>MSAASWSHPQFEKMSRDEVEALIQEVLEVYPEKAKKDRAKHLAVNDQSVEQSKKCITSNKKSLPGVMTIRGCAYAGSKGVVWGPIKDMIHISHGPVGCGQYSRAGRRNYYIGTTGVNAFVTMNFTSDFQEKDIVFGGDKKLAKLIDEIETLFPLNKGISVQSECPIGLIGDDIEAVAKQKSAELGKTVVPVRCEGFRGVSQSLGHHIANDAVRDWVLSKRDDDDSFESTPYDVAIIGDYNIGGDAWSSRILLEEMGLRVVAQWSGDGTISEMELTPKVKLNLVHCYRSMNYISRHMEEKYGIPWMEYNFFGPTKTIESLRKIAAQFDESIQAKCEEVIAKYKPEWEAVIAKYRPRLEGKRVMLYVGGLRPRHVIGAYEDLGMEVVGTGYEFAHNDDYDRTIKEMGNATLLYDDVTGYEFEEFVKKVKPDLIGSGIKEKYIFQKMGIPFRQMHSWDYSGPYHGFDGFAIFARDMDMTLNNPCWKKLQAPWKKAESEAEAVAASA[2x];>MSQQVDNIKPSYPLFRDEEYKDMLAKKRDNFEEKHPQEKIDEVFQWTTTEEYQELNFQREALTVNPAKACQPLGAVLCALGFEKTMPYVHGSQGCVAYFRSYFNRHFKEPISCVSDSMTEDAAVFGGQQNMKDGLENCKAIYKPDMIAVSTTCMAEVIGDDLNAFINNSKKEGHIPEEFPVPFAHTPSFVGSHTTGWDNMFEGIARYFTLNYMEDKEVGSNGKINIVPGFETYLGNFRVIKRMMNEMGVDYTLLSDPEEVLDTPADGQFRMYAGGTTQDEIKDAPNALNTLLLQPWQLTKTKKFVKNTWKHEAPKLNIPMGLEWTDEFLMKVSEITGKPIPESLAKERGRLVDMMTDSHTWLHGKKFALWGDPDFVMGMTKFLLELGCEPTHILCNNANKRWKKAMEAILAESPYGANSEVHIGKDLWHMRSLVFTNKPDFMIGNSYGKFIQRDTLYKGKEFEVPLIRIGFPIFDRHHLHRQTTLGYEGAMQILTTLVNSVLERLDEETRGMQTTDYNYDLVR[2x]

Nitrogenase provides access to bioessential nitrogen via the reduction of highly inert atmospheric dinitrogen (N2) to ammonia (NH3). In all nitrogenase isozymes, H-subunits form a homodimeric reductase component (‘HH’) that transiently associates with and transfers electrons to a catalytic core. This catalytic component is a heterotetramer composed of two D- and two K-subunits (‘DDKK’ or α2β2) and contains the active site metallocluster where N2 is bound and reduced to NH3. Three previously characterized ancestral variants were targeted from phylogenetic nodes within the evolutionary lineage of Azotobacter vinelandii Nif (wild-type, ‘WT’) (Garcia et al., 2023): Anc1A, Anc1B, and Anc2.

Anc1B, by contrast, is composed of ancestral H-, D-, and K-subunit proteins. In addition, all ancestral proteins crystallized in space group P 212121, which differs from the space groups for the same proteins in A. vinelandii NifDK (i.e., WT; space group P 21), Clostridium pasteurianum Nif (space group P 21), and Klebsiella pneumoniae NifDK (space group C 2). All three ancestors showed anisotropic diffraction: 2.65–2.93 Å for Anc1A, 1.82–2.8 Å for Anc1B, and 1.82–2.42 Å for Anc2. Among all ancestors, RMSDs for all atom positions are largest between Anc1B and WT DDKK (0.36 Å; compared to RMSD of 0.50 Å between A. vinelandii and K. pneumoniae DDKK). This observation may be explained by the larger number of amino acid substitutions between the fully ancestral Anc1B complex and WT, whereas only the D-subunit contains substitutions in the Anc1A and Anc2 hybrid complexes. Furthermore, we observe that the position of the twofold symmetry axis relating the two DK heterodimers of a single MoFe protein shifts slightly between Anc1B and WT. The same was previously observed in VFe protein and FeFe protein and may reflect slight differences in the interface between the two copies of NifK. Additionally, two unique single-point substitutions in the ancestral K-subunit—K211N and G307N, specific to Anc1B—are likely to impact interactions with HH E111 in the ATP-bound state. Positioned centrally within the DDKK-HH interface, these substitutions alter the electrostatic surface of HH. In Anc1B, the substitution HH S177G is located near the interface with NifDK, with G307N in Anc1B NifK identified as a potential interaction partner.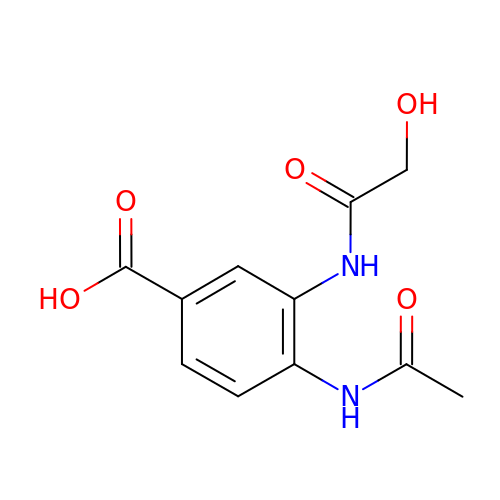4-(ACETYLAMINO)-3-[(HYDROXYACETYL)AMINO]BENZOIC ACID | C11 H12 N2 O5 | CRHJDPGLFDNPOA-UHFFFAOYSA-N> MSGDENPASKPTPVQDVQGDGRWMSLHHRFVADSKDKEPEVVFIGDSLVQLMHQSEIWRELFSPLHALNFGIGGDSTQHVLWRLENGELEHIRPKIVVVWVGTNNHGHTAEQVTGGIKAIVQLVNERQPQARVVVLGLLPRGQHPNPLREKNRRV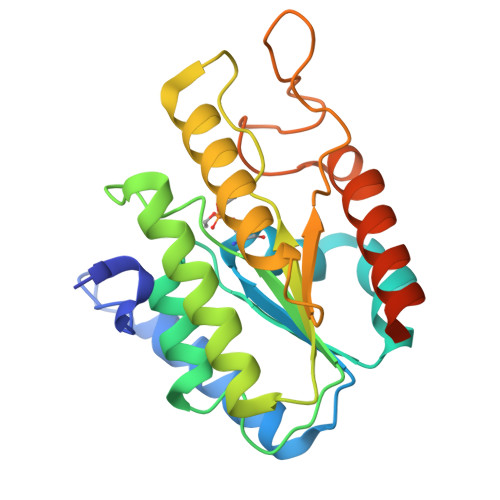NELVRAALAGHPRAHFLDADPGFVHSDGTISHHDMYDYLHLSRLGYTPVCRALHSLLLRLLTQDQGQGGAPLPEPSP> XAPKEKEVAETLRKIG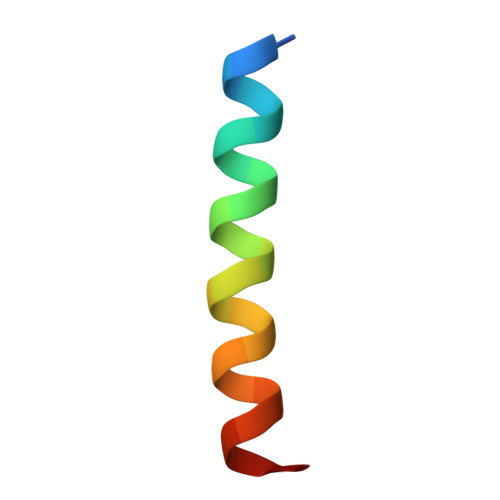EEINEALKX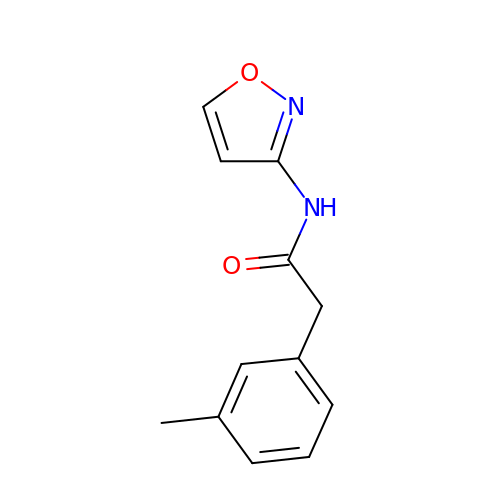2-(3-methylphenyl)-N-(1,2-oxazol-3-yl)acetamide | C12 H12 N2 O2 | AFEIJLUSZUKBHP-UHFFFAOYSA-N> FNLDTEELTAFRVDSAGFGDSVVQYANSWVVVGAPQKITAANQTGGLYQCGYSTGACEPIGLQVPPEAVNMSLGLSLASTTSPSQLLACGPTVHHECGRNMYLTGLCFLLGPTQLTQRLPVSRQECPRQEQDIVFLIDGSGSISSRNFATMMNFVRAVISQFQRPSTQFSLMQFSNKFQTHFTFEEFRRSSNPLSLLASVHQLQGFTYTATAIQNVVHRLFHASYGARRDAAKILIVITDGKKEGDSLDYKDVIPMADAAGIIRYAIGVGLAFQNRNSWKELNDIASKPSQEHIFKVEDFDALKDIQNQLKEKIFAIEGTETTSSSSFELEMAQEGFSAVFTPDGPVLGAVGSFTWSGGAFLYPPNMSPTFINMSQENVDMRDSYLGYSTELALWKGVQSLVLGAPRYQHTGKAVIFTQVSRQWRMKAEVTGTQIGSYFGASLCSVDVDSDGSTDLVLIGAPHYYEQTRGGQVSVCPLPRGWRRWWCDAVLYGEQGHPWGRFGAALTVLGDVNGDKLTDVVIGAPGEEENRGAVYLFHGVLGPSISPSHSQRIAGSQLSSRLQYFGQALSGGQDLTQDGLVDLAVGARGQVLLLRTRPVLWVGVSMQFIPAEIPRSAFECREQVVSEQTLVQSNICLYIDKRSKNLLGSRDLQSSVTLDLALDPGRLSPRATFQETKNRSLSRVRVLGLKAHCENFNLLLPSCVEDSVTPITLRLNFTLVGKPLLAFRNLRPMLAADAQRYFTASLPFEKNCGADHICQDNLGISFSFPGLKSLLVGSNLELNAEVMVWNDGEDSYGTTITFSHPAGLSYRYVAEGQKQGQLRSLHLTCDSAPVGSQGTWSTSCRINHLIFRGGAQITFLATFDVSPKAVLGDRLLLTANVSSENNTPRTSKTTFQLELPVKYAVYTVVSSHEQFTKYLNFSESEEKESHVAMHRYQVNNLGQRDLPVSINFWVPVELNQEAVWMDVEVSHPQNPSLRCSSEKIAPPASDFL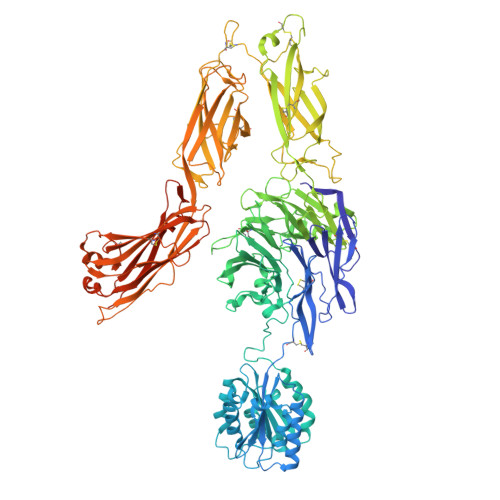AHIQKNPVLDCSIAGCLRFRCDVPSFSVQEELDFTLKGNLSFGWVRQILQKKVSVVSVAEITFDTSVYSQLPGQEAFMRAQTTTVLEKYKVHGCGGLENLYFQGGENAQCEKELQALEKENAQLEWELQALEKELAQWSHPQFEK>MMKRTFWLIALSLLSLTLSASDSLRIHNPQIPILLDRMDNVLFLIRVPDAVQGNVLESLTVEFGPDTDLNSIAELRLFYSGTEAVRRQGLRFSPVEYISAHNVWNTRSANPSYSVMQEQASKIGRKVVLHSRQPMVGGINYYWVSVRMNPDASLLTELRARVSEVVVNGKKIPVACDSREVVRRMGYGVRHAGDDHSMAYRIPGLVTTNSGSLIGTYDVRWNSSVDLQERIDIGVSRSTDKGQTWEPMRIAMSFADIDGLPSGQNGVGDPAVLVDEKTGTIWVMAAWTHGMGNG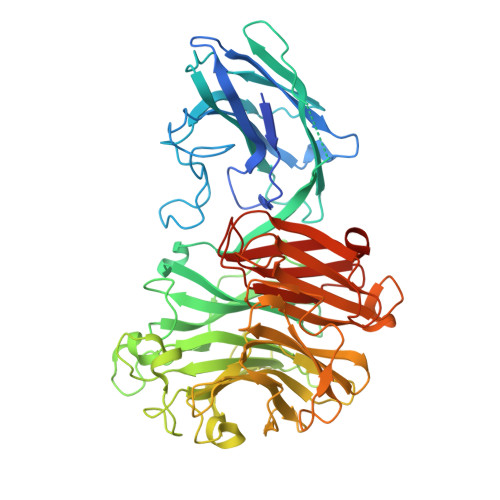RAWTNSMPGMEPMETPQLMLARSDDDGRTWSEPINITKQVKDPSWCFLLQGPGRGITMRDGTLVFAIQFIDKDRMPHAGIIFSKDHGETWHIHNPARSNTTEAQVAEVEPGVLMLNMRDNRGGARAVMTTRDLGRTWTEHVSHRTTLREPVCMASLIAVPAEKNVLGKDLLLFSNPDTTDGRRDITIKASLDGGVTWPYSLLLDEGDSWGYSCLTMIDSQTVGILYESSVAHITFQAAKLKAIVKHHHHHHHHHH[2x]>GGCUUAUACAGGGUAGCAUAAUGGGCU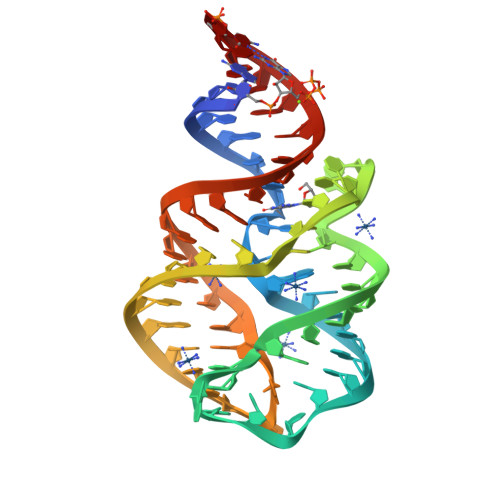ACUGACCCCGCCUUCAAACCUAUUUGGAGACUAUAAGUC[2x]[(2~{S},5~{S})-2-[[(5-bromanylpyridin-2-yl)amino]methyl]-5-methyl-piperidin-1-yl]-(3-fluoranyl-2-methoxy-phenyl)methanone 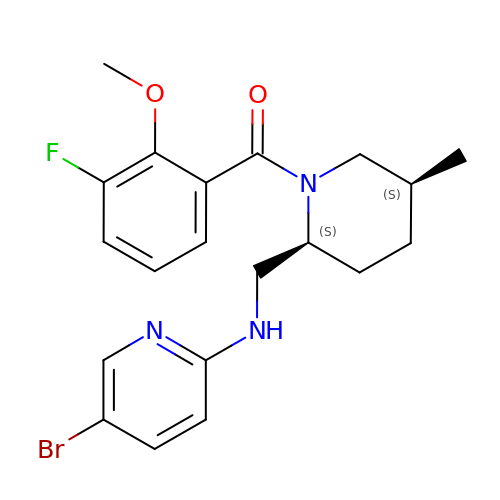| C20 H23 Br F N3 O2 | TWCRHJLMMAYSTE-ZFWWWQNUSA-N(~{Z})-2-[[2-methyl-3-oxidanyl-5-(phosphonooxymethyl)pyridin-4-yl]methylamino]pent-2-enedioic acid | C13 H17 N2 O9 P | 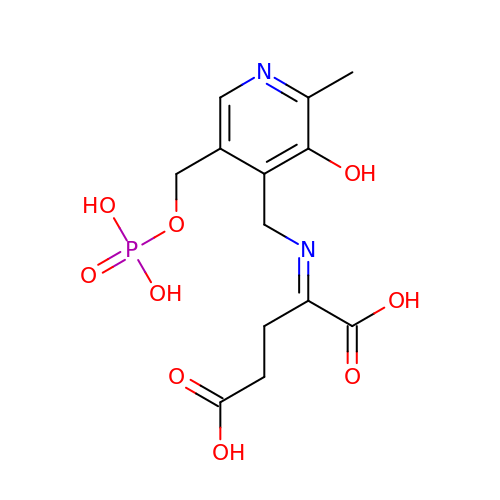AQYBBWUPMNWMHD-UHFFFAOYSA-N>SKRKIVLLMAYSGKGYHGMQRNVGSSQFKTIEDDLVSALVRSGCIPENHGEDMRKMSFQRCARTDKGVSAAGQVVSLKVWLIDDILEKINSHLPSHIRILGLKRVTGGFNSKNRCDARTYCYLLPTFAFAHKDRDVQDETYRLSAETLQQVNRLLACYKGTHNFHNFTSQKGPQDPSACRYILEMYCEEPFVREGLEFAVIRVKGQSFMMHQIRKMVGLVVAIVKGYAPESVLERSWGTEKVDVPKAPGLGLVLERVHFEKYNQRFGNDGLHEPLDWAQEEGKVAAFKEEHIYPTIIGTERDERSMAQWLSTL[2x]

One of the first identified was the pseudouridine synthase 1 (hPus1p), which is a member of the TruA family despite their low sequence similarity (<20%;). We have characterised the catalytic domain of the hPus1p protein biochemically and structurally. We determined the structure of the catalytic domain of ΔhPus1p and the D146A mutant of this enzyme. The atomic model shows the typical fold for a pseudouridine synthase from the TruA family.

Crystals of ΔhPus1p belong to space group P212121, with two molecules per asymmetric unit. The region preceding the C-terminal helices of hPus1p (residues 348–352) is described by weak electron density, and so this region was built in molecule B of the ΔhPus1p structure only. If we superimpose our structure of the ΔhPus1p enzyme onto the bacterial TruA dimer, it clearly shows that the mammalian enzyme cannot form a dimer. In molecule A, the carboxyl group of the lysine molecule forms a hydrogen bond with the backbone atoms of residue D146, while the lysine amide group is bound to the hydroxyl group of residue Y201. In molecule B of the same crystal form, the backbone of the glutamate compound is hydrogen bonded to the hydroxyl group of residue Y201, while the main chain and the side chain of residue R295 stabilise the OE1 and OE2 positions of the glutamate. The carboxyl groups of the two amino acids are located near the backbone of residue D146 and occupy roughly the same position in both molecules of ΔhPus1p. However, the glutamate and the lysine side chains are orientated in opposite directions. The side chain of the glutamate points towards residue R295 of α5, while the lysine NZ atom faces residue R144 of the catalytic loop. None of these bound molecules form hydrogen bonds with the catalytic aspartic acid D146 side chain. The presence of these two compounds with opposite ionic characteristics, i.e. positively or negatively charged, suggests that the active site cavity of hPus1p may mimic a dipole.>MCTGLRFTDDQGNLYFGRNLDVGQDYGEGVIITPRNYPLPYKFLDNTTTKKAVIGMGIVVDGYPSYFDCFNEDGLGIAGLNFPHFAKFSDGPIDGKINLASYEIMLWVTQNFTKVSDVKEALKNVNLVNEAINSSFAVAPLHWIISDKDEAIIVEVSKQYGMKVFDDKLGVLTNSPDFNWHLTNLGNYTGLDPHDATAQSWNGQKVAPWGVGTGSLGLPGDSIPADRFVKAAYLNVNYPTVKGEKANVAKFFNILKSVAMIKGSVVNKLGSDEYTVYTACYSAATKTYYCNFENDFELKTYKLDDETMNADKLITYHHHHHH[4x]

Bile salt hydrolases (BSHs) comprise a diverse family of microbial enzymes that catalyse critical BA transformation. Primary conjugated BAs synthesized in the liver, such as the tauro- and glycoconjugates of cholic acid (TCA, GCA), are deconjugated by BSHs to generate cholic acid (CA) (BA names and abbreviations are summarized in Supplementary Fig. 1). We found that Lactobacillaceae BSHs display a clear bias for either glycine or taurine-conjugated BAs. Notably, each monomer contains a loop that swaps into the active site of a neighbouring monomer within the tetramer and places amino acids proximal to the catalytic residues.

To examine the molecular foundations of BSH substrate specificity, we determined the crystal structures of six of the Lactobacillaceae BSHs examined above: four glycine-preferring (LgasBSHb, LaciBSHa, LingBSH, LreuBSH) and two taurine-preferring (LgasBSHa, LjohBSHc) BSHs. LgasBSHa structures were determined in complexes with taurine and taurine plus CDCA. We examined the sequences of these loops and found that taurine-preferring enzymes exclusively contained G-V/T-G (‘G-X-G’) motifs, while glycine-preferring enzymes solely contained S-R-G/S (‘S-R-X’) motifs. To confirm the importance of the selectivity loop, we first created two variant enzymes that swap the central residues in each selectivity loop: a V211R mutant of the taurine-preferring LgasBSHa and a R208V mutant of the glycine-preferring LgasBSHb. We found that both single-swap mutations significantly decreased the specific activities with preferred substrates without significantly impacting the non-preferred substrate. We examined the activity of LgasBSHa G23E and LgasBSHb E21G variants and found that they decreased activity with the preferred substrate without impacting non-preferred substrate activity. Third, combining these mutations by adding a G23E V211R salt bridge in LgasBSHa further lowered the preferred activity, while removing the salt bridge in LgasBSHb E21G R208V did not further decrease the preferred activity. Fourth, we created triple mutants of the selectivity loop sequence. Both the LgasBSHa-SRS and LgasBSHb-GVG variants exhibited the greatest reduction in specific activities toward their preferred substrates, with little effect on non-preferred substrate processing. Importantly, without altering secondary structure, the triple mutations significantly decreased substrate selectivity from 76-fold to 14-fold for LgasBSHa and from 353-fold to 2-fold for LgasBSHb.3,6-dichloro-2-methoxybenzoic acid | C8 H6 Cl2 O3 | 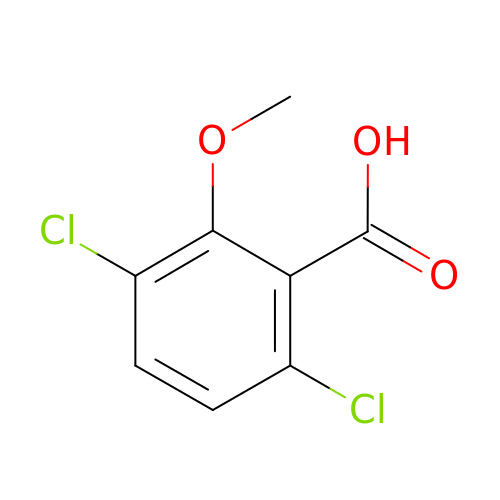IWEDIXLBFLAXBO-UHFFFAOYSA-N> MDPVLGDVIATRIYKACFKHVYGKNMKAYSEKDEAKF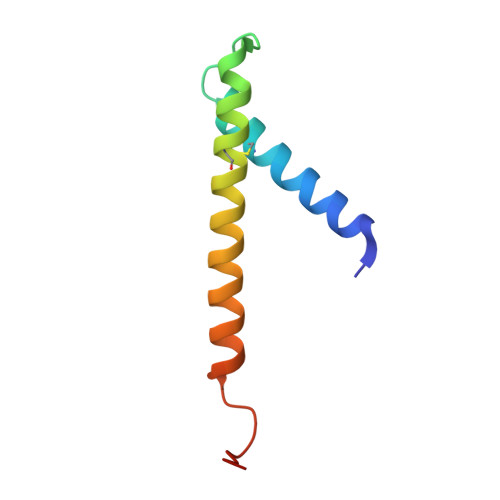DQCLTSYVESYKSVTNHFITYLGQLPKKGLSLDGS> MKTIKDRIAKWSAIGLLSAVAATAFYAPSASAHGEKSQAAFMRMRTIHWYDLSWSKEKVKINETVEIKGKFHVFEGWPETVDEPDVAFLNVGMPGPVFIRKESYIGGQLVPRSVRLEIGKTYDFRVVLKARRPGDWHVHTMMNVQGGGPIIGPGKWITVEGSMSEFRNPVTTLTGQTVDLENYNEGNTYFWHAFWFAIGVAWIGYWSRRPIFIPRLLMVDAGRADELVSATDRKVAMGFLAATILIVVMAMSSANSKYP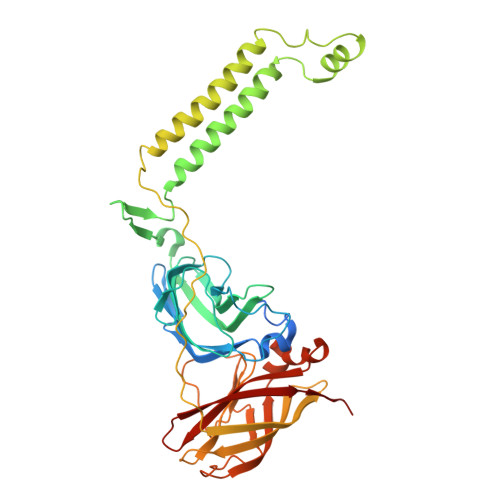ITIPLQAGTMRGMKPLELPAPTVSVKVEDATYRVPGRAMRMKLTITNHGNSPIRLGEFYTASVRFLDSDVYKDTTGYPEDLLAEDGLSVSDNSPLAPGETRTVDVTASDAAWEVYRLSDIIYDPDSRFAGLLFFFDATGNRQVVQIDAPLIPSFM1-[(2R)-2,3-dihydro-1,4-benzodioxin-2-yl]-N-methylmethanamine | C10 H13 N 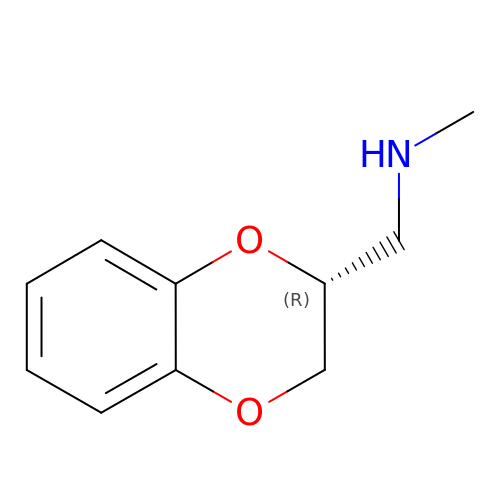O2 | RPZMFKMYOVWSQN-MRVPVSSYSA-N>[2x]MGVFMEKLKTYLELIRVKNCITASIGGIIGYLISSNFEIDILKSLLVFFVVFFVCAYGNVINDIFDIEIDRINKPSRPLPSGKIKLNEAKKFSAILLILGLVLSLFINIYALIIAVINALFLYLYAKKYKKYKPIGNFIIGYLTGSVFLFGGVAGKNVMPVVILFLCSLLSIWGREIVKDFEDMEGDKKEGVISLPIKYGKKSLYFATFLVVLAVILSPLPYILKIFGIWYLILIAICDILFIYAMAL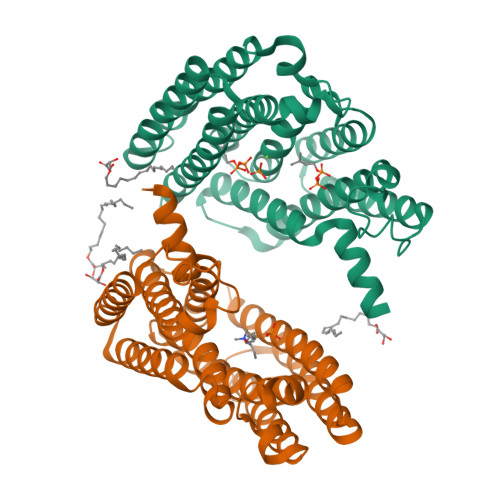LLKEPNKETASKVSKFLKIIMNIVLLAFIVGAIKL(3S,6S)-3-[(2S)-butan-2-yl]-6-[(2R)-2-methyl-2,3-bis(oxidanyl)propyl]piperazine-2,5-dion 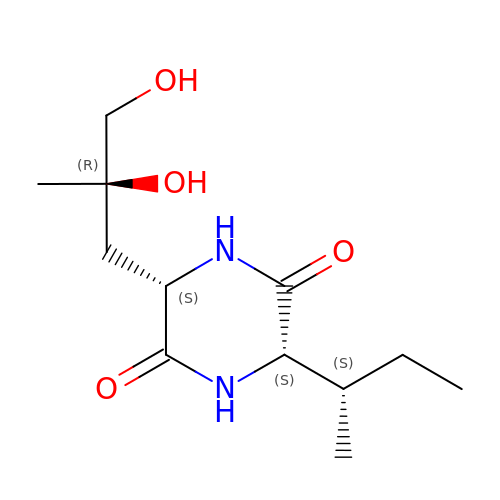| C12 H22 N2 O4 | KJJLKZILTAEYLN-PHGLEFOZSA-N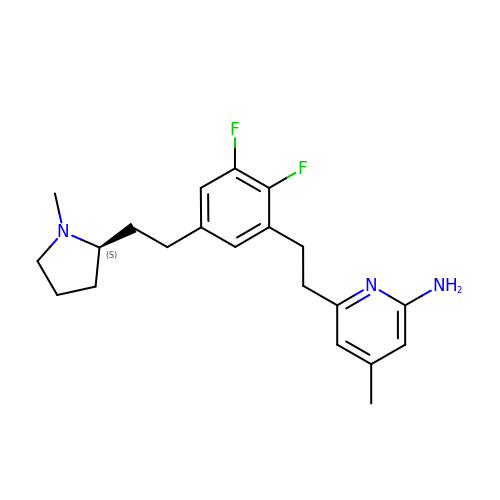6-[2-(2,3-difluoro-5-{2-[(2S)-1-methylpyrrolidin-2-yl]ethyl}phenyl)ethyl]-4-methylpyridin-2-amine | C21 H27 F2 N3 | DWIFPRVVASXUJK-GOSISDBHSA-N>[2x]MSEITLGRYLFERLKQVEVQTIFGLPGDFNLSLLDNIYEVPGMRWAGNANELNAAYAADGYARLKGMSCIITTFGVGELSALNGIAGSYAEHVGVLHVVGVPSVSSQAKQLLLHHTLGNGDFTVFHRMSSNISETTAMITDINTAPAEIDRCIRTTYVSQRPVYLGLPANLVDLTVPASLLDTPIDLSLKPNDPEAEEEVIENVLQLIKEAKNPVILADACCSRHDAKAETKKLIDLTQFPAFVTPMGKGSI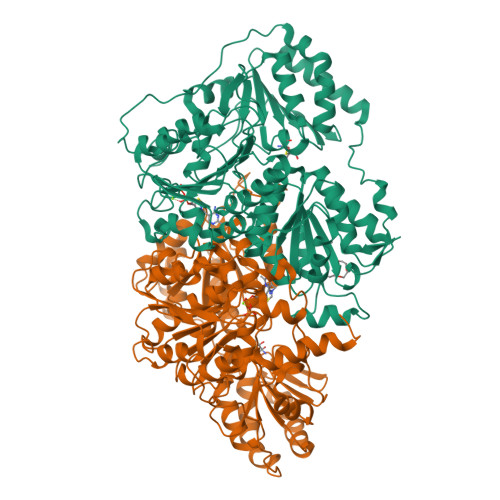DEKHPRFGGVYVGTLSSPAVKEAVESADLVLSVGALLSDFNTGSFSYSYKTKNIVEFHSDYTKIRSATFPGVQMKFALQKLLTKVADAAKGYKPVPVPSEPEHNEAVADSTPLKQEWVWTQVGEFLREGDVVITETGTSAFGINQTHFPNNTYGISQVLWGSIGFTTGATLGAAFAAEEIDPKKRVILFIGDGSLQLTVQEISTMIRWGLKPYLFVLNNDGYTIERLIHGETAQYNCIQNWQHLELLPTFGAKDYEAVRVSTTGEWNKLTTDEKFQDNTRIRLIEVMLPTMDAPSNLVKQAQLTAATNAKN>MPIVVTQAHIDRVGIAADLLDASPVSLQVLGRPTAINTVVIKTYIAAVMELASKQGGSLAGVDIRPSVLLKDTAIFTKPKAKSADVESDVDVLDTGIYSVPGLARKPVTHRWPSEGIYSGVTALMGATGSGKSITLNEKLRPDVLIRWGEVAEAYDELDTAVHISTLDEMLIVCIGLGALGFNVAVDSVRPLLFRLKGAASAGGIVAVFYSLLTDISNLFTQYDCSVVMVVNPMVDAEKIEYVFGQVMASTVGAI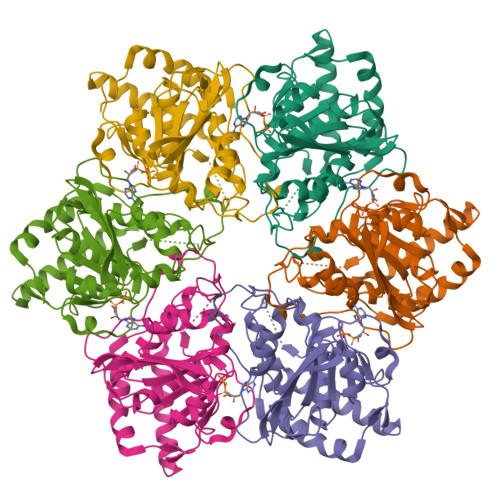LCADGNVSRTMFRTNKGRIFNGAAPLAADTHMPSMDRPTSMKALDHTSIASVAP[6x]>[2x]ISEFGSMNVILSIDQSTQSTKVFFYDEELNIVHSNNLNHEQKCLKPGWYEHDPIEIMTNLYNLMNEGIKVLKDKYTSVIIKCIGITNQRETVIIWDRITGKPLYNAIVWLDTRVEELVTEFSAKYNNNDIQKKTGTYFNTYFSAFKILWLIQNNPEIKQKIDDGTAVIGNINTWLIFNLTKGNCYTDVTNASRTLLMDINTLQWDEKMCKIFNITNMSVLPEIKSNCSNFGLVKSEHVPDYLNIPITGCIGDQQSACIGQAIFDEGEAKCTYGTGVFLLINTGEKVVYSTCGLITTICYKFNDNDKPKYALEGSIGTAGSGVSWLLKNKLIDDPSEASDIMEKCENTTGVIFVPAFSGLYAPRWR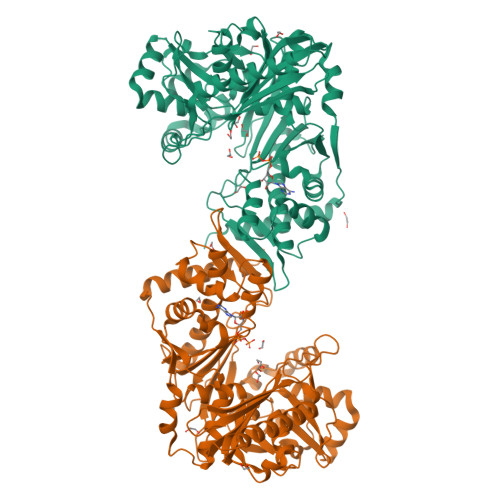SDARASIYGMTFNTERSHIVRALLEGIAFQLNEIVDSLTSDMGIEMLHVLRCDGGMTKNKPFMQFNSDIINTKIEVSKYKEVTSLGAAVLAGLEVKIWDSLDSVKSLLRRSDAVFHSKMDDKKRKKKTSEWNKAVERTLIQL4,4,4-trifluoro-1-(4-methoxyphenyl)butane-1,3-dione | C11 H9 F3 O3 | 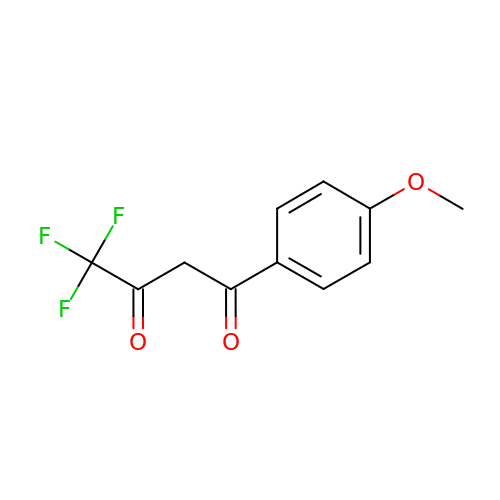NNEIYSHJFCLFES-UHFFFAOYSA-N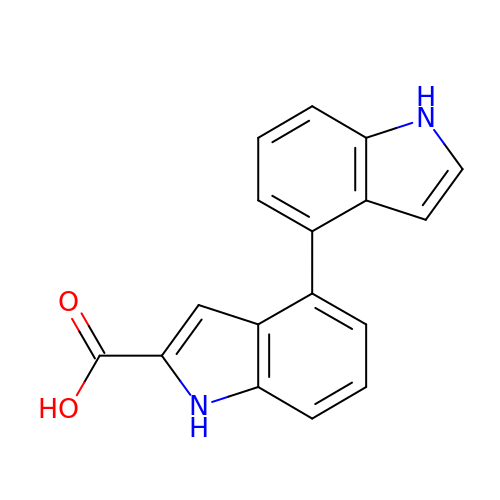1H,1'H-4,4'-biindole-2-carboxylic acid | C17 H12 N2 O2 | PXFRZQUQSWYJFD-UHFFFAOYSA-N> EDKRAKVTSAMQT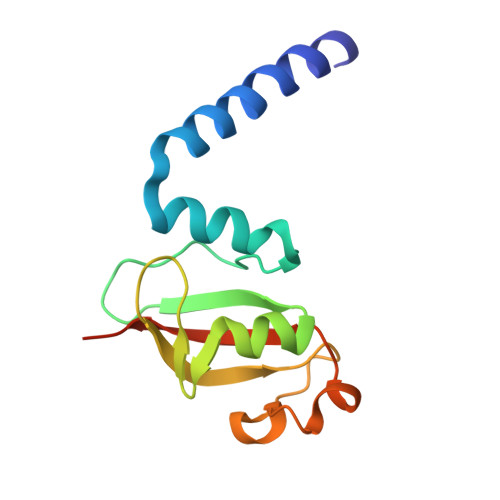MLFTMLRKLDNDALNNIINNARDGCVPLNIIPLTTAAKLMVVIPDYNTYKNTCDGTTFTYASALWEIQQVVDADSKIVQLSEISMDNSPNLAWPLIVTALRANSAVKLQ> ATDKERFIASLMARMSNAEKIGQLRLVSVGADHPKEALMADIRAGKVGAIFNTVTRPDIRAMQDQVRHSRLKIPLFHAYDVAHGHRTIF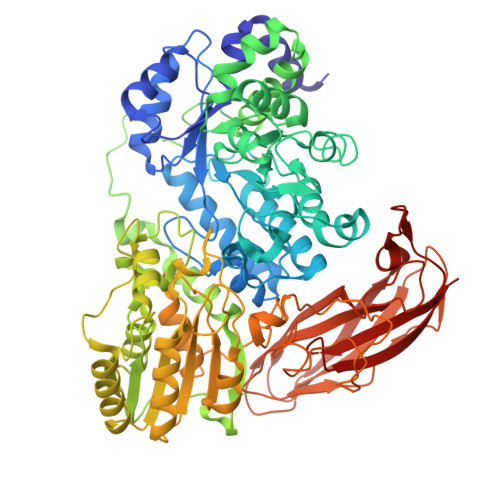PISLGLAASWDPEVVARSARISALEASADGLDMSFSPMVDITRDARWGRVSEGFGEDTYLTSLLSGVMVRAYQGSNLAAPDSIMAAVKHFALYGAAEGGRDYNTVDMSLPRMFQDYLPPYKAAVDAGAGAVMVSLNTINGVPATANRWLLTDLLRQQWGFKGLTISNHGAVKELIKHGLAGNERDATRLAIQAGVDMNMNDDLYSTWLPKLLAAGEIDQADIDRACRDVLAAKYDLGLFADPYRRLGKPDDPPFDTNAESRLHRQAAREVAREGLVLLKNRDGLLPLKKQGRIAVIGPLAKSQRDVIGSWSAAGVPRQAVTVYQGLANAVGERATLLYAKGANVSGDQAILDYLNSYNPEVEVDPRSAEAMLEEALRTARDADLVVAVVGESQGMAHEASSRTDLRIPASQRRLLKALKATGKPLVLVLMNGRPLSLGWEQENADAILETWFSGTEGGNAIADVLFGEHNPSGKLTMSFPRSVGQVPVYYNHLNTGRPMDHDNPGKYTSRYFDEANGPLYPFGYGLSYTEFSLSPLRLSSERLARGATLEARVTLSNSGKRAGATVVQLYLQDPVASLSRPVKELRGFRKVMLEPGESREIVFRLGEADLKFYDSQLRHTAEPGEFKVFVGLDSAQTESRSFTLL>MEQRASLDSEESESPPQENSCLDPPDRDPNCKPPPVKPHIFTTRSRTRLFGKGDSEEASPLDCPYEEGGLASCPIITVSSVLTIQRPGDGPASVRPSSQDSVSAGEKPPRLYDRRSIFDAVAQSNCQELESLLPFLQRSKKRLTDSEFKDPETGKTCLLKAMLNLHNGQNDTIALLLDVARKTDSLKQFVNASYTDSYYKGQTALHIAIERRNMTLVTLLVENGADVQAAANGDFFKKTKGRPGFYFGELPLSLAACTNQLAIVKFLLQNSWQPADISARDSVGNTVLHALVEVADNTVDNTKFVTSMYNEILILGAKLHPTLKLEEITNRKGLTPLALAASSGKIGVLAYILQREIHEPECRHLSRKFTEWAYGPVHSSLYDLSCIDTCEKNSVLEVIAYSSSETPNRHDMLLVEPLNRLLQDKWDRFVKRIFYFNFFVYCLYMIIFTAAAYYRPVEGLPPYKLKNTVGDYFRVTGEILSVSGGVYFFFRGIQYFLQRRPSLKSLFVDSYSEILFFVQSLFMLVSVVLYFSQRKEYVASMVFSLAMGWTNMLYYTRGFQQMGIYAVMIEKMILRDLCRFMFVYLVFLFGFSTAVVTLIEDGKNNSLPMESTPHKCRGSACKPGNSYNSLYSTCLELFKFTIGMGDLEFTENYDFKAVFIILLLAYVILTYILLLNMLIALMGETVNKIAQESKNIWKLQRAITILDTEKSFLKCMRKAFRSGKLLQVGFT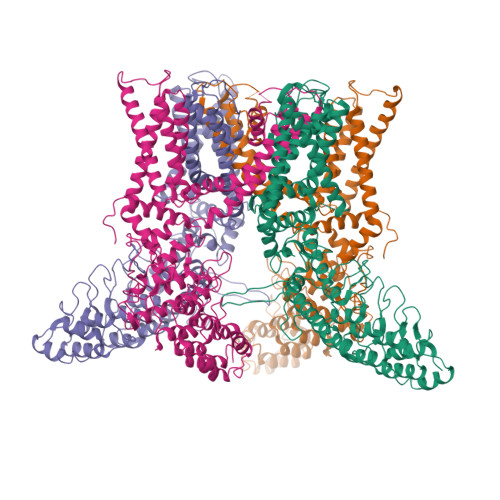PDGKDDYRWCFRVDEVNWTTWNTNVGIINEDPGNCEGVKRTLSFSLRSGRVSGRNWKNFALVPLLRDASTRDRHATQQEEVQLKHYTGSLKPEDAEVFKDSMVPGEK[4x]>GSDGDYDYLIKFLALGDSGVGKTSVLYQYTDGKFNSKFITTVGIDFREKTIYRNDKRIKLQLWDTAGLERFRSLTTAFFRDAMGFLLLFDLTNEESFLNVRNWISQLKTHAYSENPDIVLCGNKSDLEDERVVAAAEARQLAEHYGIPYFETSAANGTNISQAIEMLLDLIMKRMERSVDKS[16x]

Rab27a is a small GTPase belonging to the large family of Ras-related in brain (Rab) proteins. Rab27a is part of the secretory pathway involved in the transport of melanosomes and the secretion of vesicles containing insulin, histamine, chemokines, matrix metalloproteases (MMPs) and exosomes. In humans, Rab27a is overexpressed in multiple types of cancer, including breast, lung, pancreatic and liver cancers. Evidence supporting the role of human Rab27a (hRab27a) in multiple cancer types suggests that the inhibition of this GTPase could be a target for cancer therapy.

We therefore generated hRab27a mutants that were capable of crystallizing in the absence of effectors and were suitable for ligand-binding studies. Point mutations in hRab27a were made based on the crystal packing of mouse Rab3, the highest identity hRab27a homologue with known structure. This led to a construct, referred to as hRab27aMut, that is able to form crystals that diffract to a maximum resolution of 2.82 Å and with the potential ligand-binding sites exposed. Inspection of the X-ray data showed that these crystals were highly anisotropic, the native Patterson function indicated strong translational non­crystallographic symmetry (tNCS) and a high copy number was predicted per asymmetric unit. The diffraction anisotropy of the hRab27aMut crystals was estimated with the ANO mode of Phaser to be 207.3 Å2. To avoid these potential problems, the systematically weakest reflections with the largest relative errors were omitted from the molecular-replacement calculations. Most residues in all 16 molecules were modelled, apart from flexible residues at the N-terminus of the construct. Residues with poor side-chain density (930 out of a total of 2736 in the model) were truncated at the Cβ atom. The final refinement used a pruned data set from which reflections conveying less than 0.05 bits of information (24% of the data set) were removed. In the Rab27a structure, the SF4 pocket, formed by the α3–β5 loop (a highly variable region among Ras superfamily members) and the C-terminal region of the α5 helix, is of particular interest, as it is fundamental to the interaction of Rab27a with the WF motif of Slp2a.> TVAYIAIGSNLASPLEQVNAALKALGDIPESHILTVSSFYRTPPLGPQDQPDYLNAAVALETSLAPEELLNHTQRIELQQGAVRKAERWGPRTLDLDIMLFGNEVINTERLTVPHYDMKNRGFMLWPLFEIA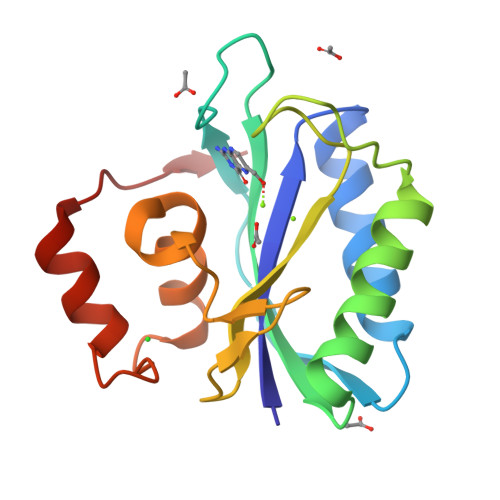PELVFPDGEMLRQILHTRAFDKLNKW> MGAQVSTQKSGSHETRNVATEGSTINFTNINYYKDSYAASASRQDFAQDPAKFTRPVLDTIREVAAPLQSPSVEACGYSDRVAQLTVGNSTITTQEAANIVLSYGEWPEYCPSTDATAVDKPTRPDVSVNRFYTLSTKSWKTESTGWYWKFPDVLNDTGVFGQNAQFHYLYRSGFCMHV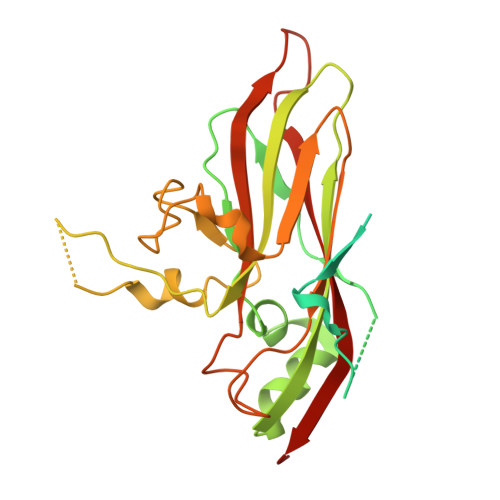QCNASKFHQGALLVAAIPEFVIAASSPATKPNGRGLYPDFAHTNPGKDGQEFRDPYVLDAGIPLSQALVFPHQWINLRTNNCATIIMPYVNALPFDSALNHSNFGLVVIPISPLKYCNGATTEVPVTLTIAPLNSEFSGLRQAIKQ> MEKVNEILSQLTLEEKVKLVVGVGLPGLFGNPHSRVAGAAGETHPVPRVGLPAFVLADGPAGLRINPTRENDENTYYTTAFPVEIMLASTWNRELLEEVGKAMGEEVREYGVDVLLAPAMNIHRNPLCGRNFEYYSEDPVLSGEMASSFVKGVQSQGVGACIKHFVANNQETNRMVVDTIVSERALREIYLRGFEIAVKKSKPWSVMSAYNKLNGKYCSQNEWLLKKVLREEWGFEGFVMSDWYAGDNPVEQLKAGNDLIMPGKAYQVNTERRDEIEEIMEALKEGKLSEEVLDECVRNILKVLVNAPSFKNYRYSNKPDLEKHAKVAYEAGAEGVVLLRNEEALPLSENSKIALFGTGQIETIKGGTGSGDTHPRYAISIL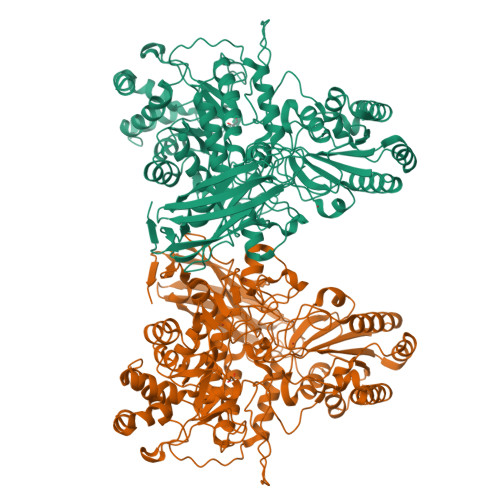EGIKERGLNFDEELAKTYEDYIKKMRETEEYKPRRDSWGTIIKPKLPENFLSEKEIHKLAKKNDVAVIVISRISGEGYDRKPVKGDFYLSDDETDLIKTVSREFHEQGKKVIVLLNIGSPVEVVSWRDLVDGILLVWQAGQETGRIVADVLTGRINPSGKLPTTFPRDYSDVPSWTFPGEPKDNPQKVVYEEDIYVGYRYYDTFGVEPAYEFGYGLSYTTFEYSDLNVSFDGETLRVQYRIENTGGRAGKEVSQVYIKAPKGKIDKPFQELKAFHKTRLLNPGESEEVVLEIPVRDLASFNGEEWVVEAGEYEVRVGASSRNIKLKGTFSVGEERRFKP>[2x]MKKWSDT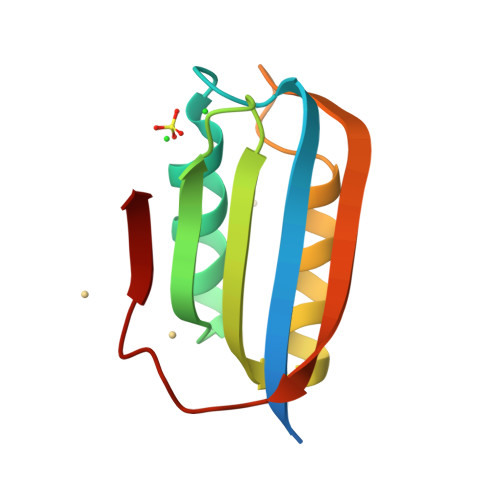EVFEMLKRMYARVYGLVQGVGFRKFVQIHAIRLGIKGYAKNLPDGSVEVVAEGYEEALSKLLERIKQGPPAAEVEKVDYSFSEYKGEFEDFETY>[2x]MTAVVKNLAKLPAATSQILTNVSKLQTFHGLLEERRDKYAPLAYHTYDNLKQKTTWHPIAHAWVDEGLPVSKKEYNEYCWLKKDMQRLLPLASPFVFGIYGILPLAVWLSNDGYLPSAFSSKKDIVSKKLEWYSSYGDDLRQQVGPMLQHRLKRHLRGTLNNEHRLMLDEVTESYKEIFYSHYTGQLRDVRKCAHLRLYDGTSTVLLLTNKEPVELTSELLQKWNAIKAAKLSPEEEKKARNEALIEAYKEQELHGGPHVKHMQGYGIPADTPLLGENAKGDQYTQPPESASIPLEQLEWTGDTVFIPAEYRTEMEDWGRELTKLANQFLLLPWRFVSNAWNQRRLVSWFEEILQEDALIAKEGGVQALSDDELKVALLDRAVIRCDEELTRGDMEARYKEISWLMSLRNPFIVLAWQTGYYRSTYSPEDDLPEASILPKLNRTVLDVDVHNELAPDHPEKPLPRVHPALYPNSHLALAKEVAVLAK;>[6x]MHYAEAATPAKSAGSAVAKKHLEAKQKIGFVHGIDGTIATIAPAASKVTVPYNTVLEIAVSATNIANALVFNLEKDGSIGVILLDNISEVRSGQDVYATGSLLKIPVGFHMLGKIINPLGKEIPTGLFTKAAPLLDDTKLGLVEEMAPNIVSRQPVNYNLLTGYKVIDTLIPVGRGQRELILGDRQTGKTSIALSTILNQTKVNNEILSKNNVLSVYVSIGQRCSNVARIHRLLTEYDAMKYCTIVAATAADPAGLQYLAPYAGTTLGEEFRNSGRHILLVYDDLSKQAVSYRQISLLLRRPPGREAYPGDVFYLHSRLLERSAMMSPQKGSGSLTSLPIVETLSNDVTAYIVTNVISITDGQIYLDAKLFTGGQRPAVNIGLSVSRVGSSAQNKAMKKVGGALKMLMGEYRKMAGEQTSGSQNVSPVMIRGARCLQLFNQKGPSYFMDAIVALYAVTNGYMDDVKLQYSKFYEFLLLNKDLPVLYGQVNNKYFYMYNKNLNYFIRYFGLNHEILEPELKKYIEIHTNLFLDNYQSRMNELKSDEDLVQLKNLLYACKRTV;>MVGRMMATAPATAADVKQVGYVQQIIGAVVDVTFTDSVPPVLTALTVDAKETGTLLTMEIVQHLDTKTARCICMSSTDMLRLRTPVVNTGSQITVPVGEATLGRIFNVMGDAIDQRGPVKNKVRWPIHRKAPTLAEQSGKDEVLVTGIKVIDLILPYCKGGKIGLFGGAGVGKTVIIMELINNVAKGHGGYSVFAGVGERTREGTDLYLEMMGSKVIDLQGDSKCVLVYGQMNEPPGARARVAQTALTMAEYFRDEAGQDVLLFVDNVFRFTQANSEVSALLGRIPAAVGYQPTLAEDLGMLQERITSTVKGSITSVQAVYVPADDITDPAPATTFSHLDATTVLSRSVAEAGIYPAVEPLECASRIMDPDAIDVNHYNVAMDIVEMLTKYKELQDIIAVLGIDELSEEDKLIVDRARKVAKFMSQPFAVAEVFTGMKGYYVQLEDCVSDFGSLLMGQCDNIPEMAFYMVGGLDSVKEKAAKMAAEAAAMRERARKAAEAK[6x];>[2x]MPGGGTIRFWREKLEGYKKYHQIVKTIKMVTLAKYRQTVVRTRVRDQTLRYTRKALDAKTQDDQEVIEKSECLLYVPITTNRGSCGALNTNMVRYLQEVENPKMTIISVGKKALDAMTKVFQDTYRRTILNDMKQAMSFQFAAYVLEHMNTVPWDRAQIVYNRYHGAASQKLAIFNLPKFEDWKQKLEEDSAGDGKIEEDGLLQSLPMKTALGELEETAVEDFYNFHSCLAVLNAVSENELSEYAARIVAVENQLGNITGLMQLADYTYNKTRKELITAELLEIIGTMTAMHAGKKVGLKKTEFWK;>[2x]MRASRTLLLSVSRFMRQDPRKFFPDNGFRFFDGPEDSFGDGNIPAQIILTLTRQDEFILKQEPVAAITIRTNEGEMGVLAGHEYTVQQLAPGILEVEYEGGKKDQYVISGGFAHVNDTGVVDINTVEAVPLEEIDHEKLAKALEEARAKSQSPDEAVRIQGEIALEIFEPLEAALH;>MSWRDAGISYLRYLSIVTRCIHEVQKEGPLLTKNVRFSTIGWKSLYLDHGATKEYTAIPAELEKIPENQVAQQHHA[2x];>MQKLSRVVCNRLVRFHGTVAASAGGKRYDLFGYEVSVATGPFIEEIKKAQFYDDAGEVIVKMNLANTPPDLQTYNAVLERILNCKSKRSQPVKGENKFAAMMDILEEMDARSGIKPNAESWGYVLKELVQAGDFRLGWVCIAGMKSLGITPDQALVDANEANAAKAKAAGTDFPAYLKKAAPESFDTKAWGI[6x];>MHMRRAVSVFGRCRSLNGLRNYAVPSPKYIEIYQSDFSRNAYPLELLGGSHVDFAKLLYSFADQVENKKFEVYVEDFKKLDSIIAEKGPFWAEEKIFQSPTFQGLSEGFKFILGWIQSEGAIDRLENVRLAYKELVNEARKETTATVIVAKEPSGNDLAEIRKQVEELHKESPLKDYKLVLETKVDPSIGGGYILEVCNQVVNRSAAAAAAETAALAKASAAQVDWTSLPAAPPRPSPSAPDTLIRLLGSVVDDLADADKVEQKYGA[2x];>MAAACAVRGFTTARPMLTPNKVKVPGRKPQDEEDLTWAEADRKLTPEERYARDKQMALLDKMTSQVEELEKSHTEQKKSNKGVKAQIEAISRQLEALKAQLKE[2x];>[20x]MQRGSSITKVVRRAALARSTRNAAIAYEVTVNGANLIGAGMAASGVGVPAIGVAMCFSSYMLAAARQPNMSAKLLPYCILGFALSEALALFTLLIALLELFVFS;>[2x]MAAKTIPFVASTALGERLFAGVQKVLAAAKAPVSLVQTDAKFAPADAKYLLAEPLSAAATGELANKYGLSSKVTSGAASQFYPNSIYPSLNVEVVQNLYALSNPAFSSLSATTTKAVTVKDESAIKLAELQKETERNISSFFRDEANKSVQATLRLACDKAIKTKADKKTVMVVTKPHGDAFDDLLAQVTKSESDGRADELRNSSVSVEPTLVGNAWPKLVMFPEGVNVVVCGPNASGDQVAQLFVGIAGGTGMVAQQLVGDAVVFTSANAEDNENPTGALLAASNLLTALGHEAEAKKIAAAVAKAYTTDRILPKELPGGKADLEAFIDAVAKHASA;>MFRGFRPVLAADAVKFQTLYNVLTGKQHLKDQVPVKDCNLTAIFGASWKADLNKWFDSEYAPKLPAAERDSAKKSLDLYLKRVDLTRYTREELTTYGILACGPGKVDALTEKHLLETGKARLEELTAGLGNKDEGVNAFRKEVEQEGKYANWPAEKSKALADKVIAASP[2x];>MTHAELHLFDLDEFMQTYKRLQTRQDWLIENKCKKSRLFSYVAAVIAFTVGKSATMSDEAILAKIDPYVTSEVRVQRGAWWRSGYFTKEEVEMMTPKGPIARYYKFLLGVRRFPLKHGALSWACGFVPAWLTFTSLNHWAQNRRLNRYLTQESVFGEMARELVRGKTADEATTSVMARVEKEILGVH[2x];>[2x]MSSYTGAALAPKSERLRLAFEEKQKDHQKCIEEAKGKGLKKDELIDACAWTHRKTILALKDWFAYRPPFQDRRSKWAEYCSIRHDSGSW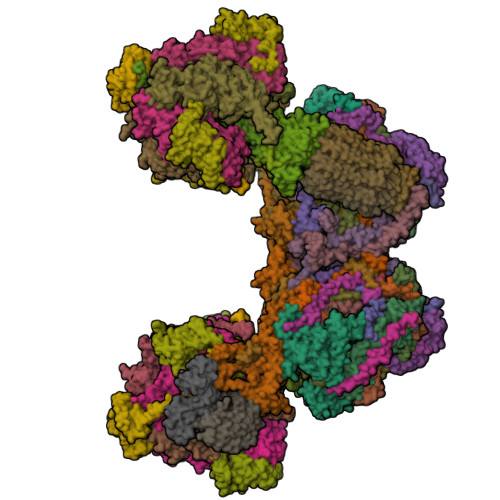LGWSQKFF;>MLNSNIYIIIYGGIIMYSIMIIIQMFLYNFSNKIYIEVEINKYILSKNNIDIYWIICNCTIIIIITTLNHIINKIGIYNMIEYNICYWLIGTGLGLYISPFIVFGYKFFVYIMDLNNYSLNIYHNNNKMNDIQQIYNGTNYNDTMIFFIKDINNIFTIYRSINFFMNWLYQMIYYGVRMWLVFVLHSFSLGSFGELITVITDNNLIFNVFYIGLLGLGFILYLIVIFYLGIQIYVYISFSLSFLHSTILLFLVNYIPHYNNKSIFNTFTNKSIY[2x];>[2x]MPSTSPADKDVPMSILHTHGLSYVNWCMSLAPGLLVFEGFFRARYYRSRVPPSRTVLMNGLKMRMFSLARQQAPKIVHKPVLSPIPEHLRLVKNVAQVQIDMLKLLNAQAAK;>MMRRACRIIRPSHVRGVSGVAPTIYLRSKAALPATSTTDVRPQLYALQRFAKAQLKTATEAERAAIEADIARYQEYLDSDLEKLKQDVAEDTAKKQKLIPLLDRYPDVPIEKIPEHANVLLKKIDACLEILSKDIGEVTDAEAHEMYFETSKFQILHIYTGCVASFPEGDVPPGAVECLPGQVIRTKVNGEDVMLEIDEVDPGYQVCWFKPDVPLPENAEILWSYPYEPTAALPTGTTWEEGQANVLIPAEPTPEAAVWPPTPVTNVYAPMAEKLALKSNPELKVLFKEALLQPAKLLPLDVDYQCSHDREVVEAKRDRYLTALVEAEQAPPLPFTPDVLQLQLEHNVLKGELIDRLRALEYTIVTEQLQARLHERRLRGDVIDEWEELDYHPLVRDDTYLAIDFGDPTFGRYIWKLFPHTDGDEECMFKDTRLDVLPPQVNPLNAILAQHTAQTPVHRSLEKRLWTEVRATAVSE[2x];>MAPLYPVLSQASLYKRHFFKNIKLFHVVFYVGAPCVTFGTAAWSGSNRNSREAIFMVIEERHGWDNFKKLSSHQQGVIMQEAAQESLLARNKGELHLP[2x];>MVYTNWQSSYTRLFVSKPWMWHPLAWMTLSVGIWWKFGKESLCNERSFYIHTHPKWAPHKFHTVYNWSRDPIKWTLAEQYASIIRNTNTDIEAVLKIKLPANAN[2x];>[2x]MAFGRTRPTLSSPLVPVWNDLRALQVFTSQEYMQKRGPGFTNTLEYKLSCLNPVKWYDMMKVMPGGKAFVGTALGLALFGGWGVEFVKNISVMTKEKPPIDWNNEKLGHLTRS;>LIPVSLVDLININIIFYILLLYTLLLFFIPLFLASINYTYHYIYKYYNYNYNFINNN[2x];>MSLAKVWMYASWIPRGIPKAMANELSSAAAALAHPEAIARVAQLESQGKNPYRVARAEFWQMYLACWPYRFRNTVVEWETCKAKVLKGSVDLQDIVDLLYLLAWAYLFWILGEIYGRGSLYGYRFDGEIHRQEAQNVILYKEKEAQEMAVVMEKLEKEIQEWLKTMEQE[2x];>[2x]MPLPNAVVQGYTSVRGPKRPLDHFYGRTPLNIDTLWHWVKFPHRYDNLRFAVCFWAFLVSAHFANKKQRNLRVEWEKNMEIQKKLHPSGLWSEEQAFAAAEKLGRPKAGHPMRVFEDGYQQFDLKPKLFDPDEEAHH;>MADHNKKDVGSWASPNEHLMFFDFSSWLLVDFGKRWERWVSFKKSFLTTTRSPYWSPQFFLLTFFQLRNSNVKLCENWNWAPKGDDFNLLHNSAAEPFGRDLKAHLEREAGAKHHH[2x];>[2x]MGGDAHAAPAEKPDPALDATKALPKALEEVEFFQSYAVRRKTGFHLFNRATGSPTIVGPMFYNLYNFVRIGRVSKYVCWLSLPLVFQRMWMKNRATGMEYDIDLENYAPFEAKKNPMHGH;>[2x]MSLPTFFLAPPLTEPFRARHRRKCIEKKDTFFQCLDKNKNETEPCEVEASGYSQECPDSWRRYFNEQRWKALELKGEVKHANLKNTQQHF;>[2x]MFGVTRKLLGELSEYVEVNEKGMPKPQALSLWNMPYAKRRALTKFARGVRWQFIVLFIALYNFKNRDDSHLLRRGAYN;>[2x]MMRISRKLLVPVANFRPKKPWDGPWGIQISQKKDRPFIAMWILFPLLLVDHLTREYYAYWHSSKVPVTDVFGDF;>[2x]MGGKASEAVTIAFRFPHRTTFLVKQNVGQKLNKGHQTFWQLVAGGWLFFLLINRTSFKPKLAAPKV>[4x]MALSMTGGQQMGRGSMSRDPLPFFPPLYLGGPEITTENCEREPIHIPGSIQPHGALLTADGHSGEVLQMSLNAATFLGQEPTVLRGQTLAALLPEQWPALQAALPPGCPDALQYRATLDWPAAGHLSLTVHRVGELLILEFEPTEAWDSTGPHALRNAMFALESAPNLRALAEVATQTVRELTGFDRVMLYKFAPDATGEVIA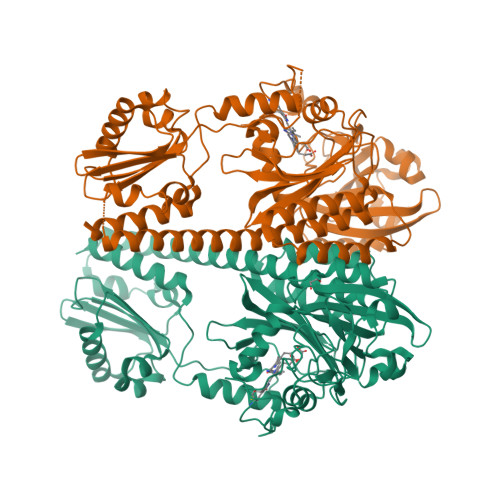EARREGLHAFLGHRFPASDIPAQARALYTRHLLRLTADTRAAAVPLDPVLNPQTNAPTPLGGAVLRATSPMHMQYLRNMGVGSSLSVSVVVGGQLWGLIACHHQTPYVLPPDLRTTLEYLGRLLSLQVQVKEAADVAAFRQSLREHHARVALAAAHSLSPHDTLSDPALDLLGLMRAGGLILRFEGRWQTLGEVPPAPAVDALLAWLETQPGALVQTDALGQLWPAGADLAPSAAGLLAISVGEGWSECLVWLRPELRLEVAWGGATPDQAKDDLGPRHSWDTYLEEKRGYAEPWHPGEIEEAQDLRDTLTGALEHHHHHH> IAKNDFSDIELAAIPFNTLADHYGERLAREQLALEHESYEMGEARFRKMFERQLKAGEVADNAAAKPLITTLLPKMIARINDWFEEVKAKRGKRPTAFQFLQEIKPEAVAYITIKTTLACLTSADNTTVQAVASAIGRAIEDEARFGRIRDLEAKHFKKNVEEQLNKRVGHVYKKAFMQVVEADMLSKGLLGGEAWSSWHKEDSIHVGVRCIEMLIESTGMVSLHRQNAGVVGQDSETIELAPEYAEAIATRAGALAGISPMFQPCVVPPKPWTGITGGGYWANGRRPLALVRTHSKKALMRYEDVYMPEVYKAINIAQNTAWKINKKVLAVANVITKWKHCPVEDIPAIEREELPMKPEDIDMNPEALTAWKRAAAAVYRKDKARKS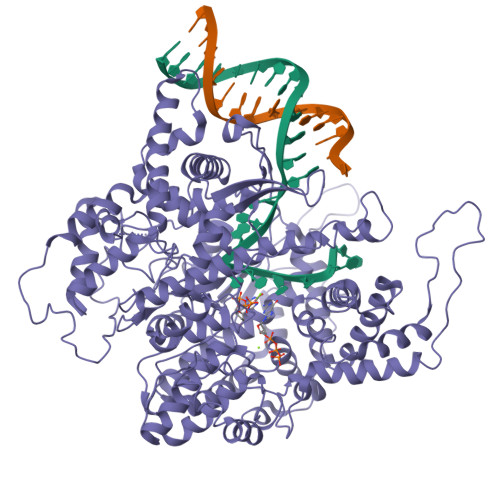RRISLEFMLEQANKFANHKAIWFPYNMDWRGRVYAVSMFNPQGNDMTKGLLTLAKGKPIGKEGYYWLKIHGANCAGVDKVPFPERIKFIEENHENIMACAKSPLENTWWAEQDSPFCFLAFCFEYAGVQHHGLSYNCSLPLAFDGSCSGIQHFSAMLRDEVGGRAVNLLPSETVQDIYGIVAKKVNEILQADAINGTDNEVVTVTDENTGEISEKVKLGTKALAGQWLAYGVTRSVTKRSVMTLAYGSKEFGFRQQVLEDTIQPAIDSGKGLMFTQPNQAAGYMAKLIWESVSVTVVAAVEAMNWLKSAAKLLAAEVKDKKTGEILRKRCAVHWVTPDGFPVWQEYKKPIQTRLNLMFLGQFRLQPTINTNKDSEIDAHKQESGIAPNFVHSQDGSHLRKTVVWAHEKYGIESFALIHDSFGTIPADAANLFKAVRETMVDTYESCDVLADFYDQFADQLHESQLDKMPALPAKGNLNLRDILESDFAFA> DVYQEPTDPKFPQQWYLSGVTQRDLNVKAAWAQGYTGHGIVVSILDDGIEKNHPDLAGNYDPGASFDVNDQDPDPQPRYTQMNDNRHGTRCAGEVAAVANNGVCGVGVAYNARIGGVRMLDGEVTDAVEARSLGLNPNHIHIYSASWGPEDDGKTVDGPARLAEEAFFRGVSQGRGGLGSIFVWASGNGGREHDSCNCDGYTNSIYTLSISSATQFGNVPWYSEACSSTLATTYSSGNQNEKQIVTTDLRQKCTESHTGTSASAPLAAGIIALTLEANKNLTWRDMQHLVVQTSKPAHLNANDWATNGVGRKVSHSYGYGLLDAGAMVALAQNWTTVAPQRKCIIDILTEPKDIG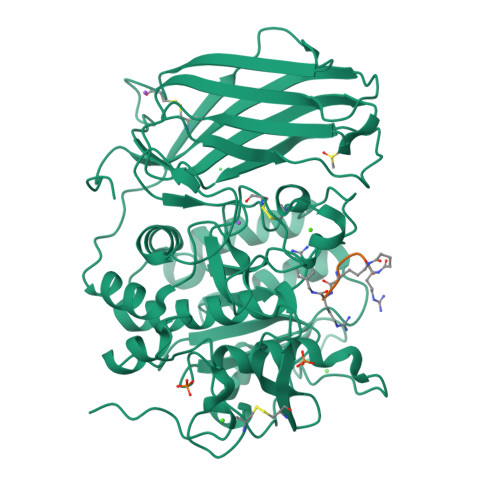KRLEVRKTVTACLGEPNHITRLEHAQARLTLSYNRRGDLAIHLVSPMGTRSTLLAARPHDYSADGFNDWAFMTTHSWDEDPSGEWVLEIENTSEANNYGTLTKFTLVLYGTASGSLVPRGSHHHHHH;> RRRKRX>[2x]QTEQGANISDQWTGSELPLAFASDSNPSDPVSNVNDKLISYNNQPANRWTNWNRSNPEASVGVLFGDSGILSKRSVDNLSVGFHEDHGVGAPKSYVIEYYVGKTVPTAPKNPSFVGN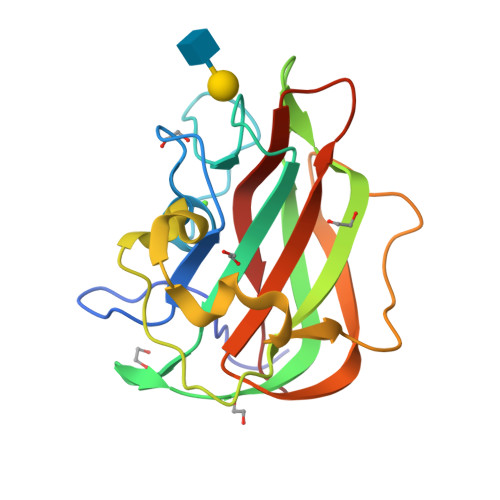EDHVFNDSANWKPVTNLKAPAQLKAGEMNHFSFDKVETYAIRIRMVKADNKRGTSITEVQIFAKQV>MGSSHHHHHHSSENLYFQGGGHMMHVLIVSDNKPLVSFIQNLVAVNADKFQSVTFDYRYSAINK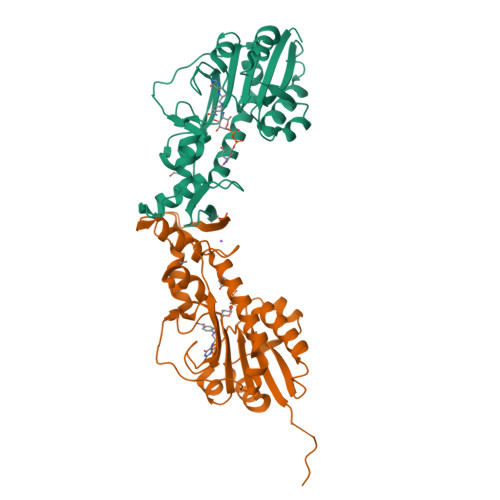NPASLISLGLTSINVKSEKDVAHIVEHYELVVSAHCKQIFPSELVNNVRCINIHPGLNPHNRGWFPQVFSIINKKPVGCTIHLMNEEIDDGAILFQKEVPIFEWDTSLNVYERVQQTEMDLLKDHLADLVFANYQQKLSYEKGNYNGISDFKALCKLNLDHIGTLRDHIDLLRALSHGDFNNAYYLRPDGSKVYIRLSAELVK[2x]> MANVMKAPRRQLTYVTDLNKCIGCQTCTVACKKLWTTGPGQDFMYWRNVETAPGLGYPRNWQTKGGGYKNGELQKGKIPPMIDYGIPFEFDYAGRLFEGKPGRVRPSPTPRSAPNWDEDQGAGEYPNNSFFYLPRMCNHCTKPACLEACPNEAIYKREQDGIVVIHQDKCKGAQACVQSCPYAKPYFNPLTNKANKCIGCFPRIEQGVAPACVAQCVGRAMHVGFVDDVNSSVYKLIKQYKVALPLHPEFGTEPNVFYVPPVLGPRIEMANGEPSTDPKIPLAQLEGLFGKQVRDVLAILQSEREKKMKGLASDLMDVLIGRRSTDMMI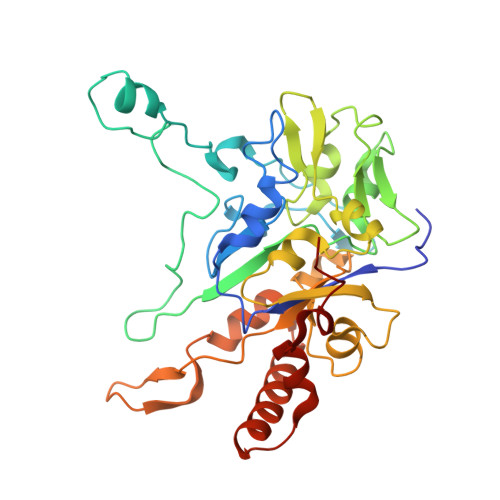SPLT>[4x]AMP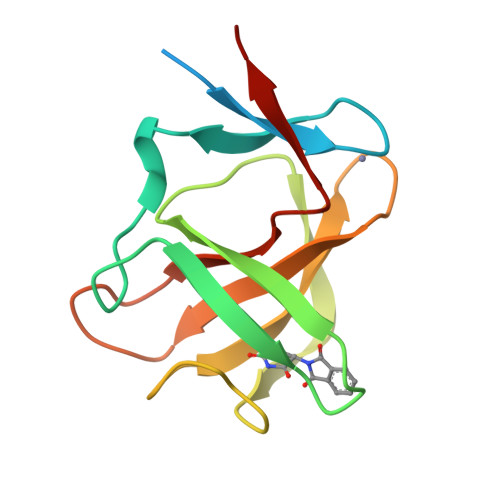LDAGGQNSTQMVLAPGASIFRCRQCGQTISRRDWLLPMGGDHEHVVFNPAGMIFRVWCFSLAQGLRLIGAPSGEFSWFKGYDWTIALCGQCGSHLGWHYEGGSQPQTFFGLIKDRLAEGPAD> NECISVKGRIYSILKQIGSGGSSKVFQVLNEKKQIYAIKYVNLEEADNQTLDSY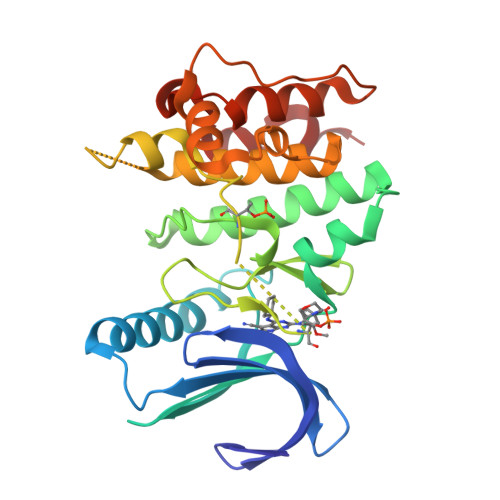RNEIAYLNKLQQHSDKIIRLYDYEITDQYIYMVMECGNIDLNSWLKKKKSIDPWERKSYWKNMLEAVHTIHQHGIVHSDLKPANFLIVDGMLKLIDFGIANQMQPDTTSVVKDSQVGTVNYMPPEAIKDMSSSRENGKSKSKISPKSDVWSLGCILYYMTYGKTPFQQIINQISKLHAIIDPNHEIEFPDIPEKDLQDVLKCCLKRDPKQRISIPELLAHPYVQIQT>[2x]GPLGSMQYVGPYRLEKTLGKGQTGLVKLGIHCVTCQKVAIKIVNREKLSESVLMKVEREIAILKLIEHPHVLKLHDVYENKKYLYLVLEHVSGGELFDYLVKKGRLTPKEARKFFRQIISALDFCHSHSICHRDLKPENLLLDERNNIRIADFGMASLQVGDSLLETSCGSPHYACPEVIRGEKYDGRKADVWSCGVILFALLVGALPFDDDNLRQ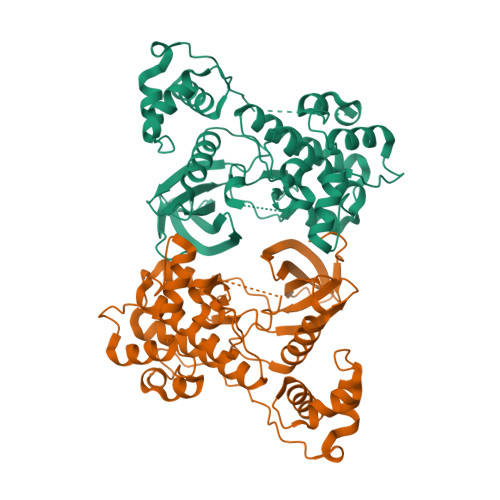LLEKVKRGVFHMPHFIPPDCQSLLRGMIEVDAARRLTLEHIQKHIWYIGGKNEPEPEQPIPRKVQIRSLPSLEDIDPDVLDSMHSLGCFRDRNKLLQDLLSEEENQEKMIYFLLLDRKLEHHHHHH> KETAAAKFERQHMDSSTSAASSSNYCNQMMKSRNLTKDRCKPV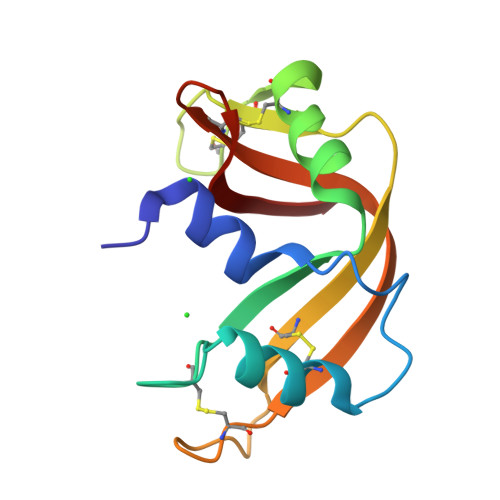NTFVHESLADVQAVCSQKNVACKNGQTNCYQSYSTMSITDCRETGSSKYPNCAYKTTQANKHIIVACEGNPYVPVAFDASV>[3x]MDNYQELRVQFAAQAVDRNEIEQWVREFAYQGFDARRVIELLKQYGGADWEKDAKKMIVLALTRGNKPRRMMMKMSKEGKATVEALINKYKLKEGNPSRDELTLSRVAAALAGWTCQALVVLSEWLPVTGTTMDGLSPAYPRHMMHPSFAGMVDPSLPGDYLRAILDAHSLYLLQFSRVINPNLRGRTKEEVAATFTQPMNAAVNSNFISHEKRREFLKAFGLVDSNGKPSAAVMAAAQAYKTAA

The N protein is the most abundant viral protein in the Phlebovirus virion and plays a key role in encasing vRNA in a protective coat. In addition to its critical role in protecting the vRNA and the antigenome (cRNA), the N protein also plays an active role in RNA transcription and replication, as well as in virion assembly. Here, we present the crystal structure of RVFV N forming a hexameric ring. In conclusion, the structure of the hexamer formed by the RVFV N protein presented here shows that oligomerization is mediated by a flexible N-terminal arm, which binds a hydrophobic pocket in the adjacent subunit.

& A resolution cutoff of 2.3 Å was chosen to retain only the most reliable data for phasing purposes. Hexamers I and II in the crystals of the native protein superimpose very well, but the two rings in the crystals of the selenomethionyl protein are slightly different. While hexamer II formed by seleniated N is the same as the two hexamers formed by native N, the subunits in hexamer I are more closely packed about the 6-fold symmetry axis. The domain of N that is near the center of the ring, comprising the loop connecting helices α10 and α11, occludes part of the central aperture, suggesting a twist in the assembly of the ring subunits. Superimposition of native and seleniated hexamers I based on subunits A, creates an 11° deviation between the planes of the two rings. Furthermore, comparison of the subunits in hexamers I formed by native and seleniated protein shows that the contraction of the ring is due to a lateral slippage between adjacent subunits. The different hexamers seen in our crystals and the variability in the oligomeric state of N-RNA complexes seen in EM images demonstrate substantial flexibility in the interaction between subunits.>[2x]ALAKRIDAALILKDGRVVKGSNFENLRDSGDPVELGKFYSEIGIDELSFWDITASVEKRKTMLELVEKVAEQIDIPITVGGGIYDFETASELILRGADKVEINTAAVENPSLITQIAQTFGSQAVVVYIAAKRVDGEFMVFTYSGTK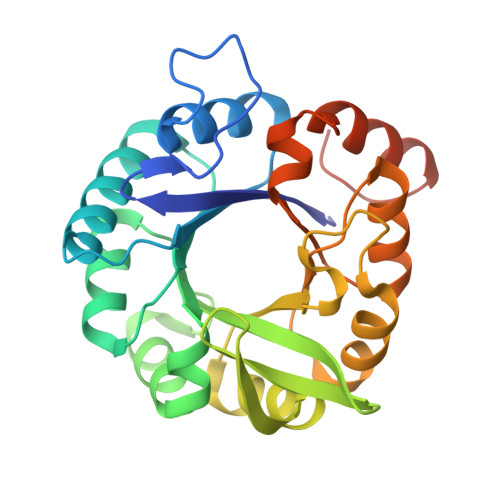NTGILLRDWVVEVEKRGAGEIVLGSIDRLGTKSGYDTEMIRFVRPLTTLPIIAHRGAGKTEHFLEAFLAGADAAKADSVFHSREIDVRELKEYLKKHGVNVRLEGLGSLEHHHHHH> TQAKAKHADVPVNLYRPNAPFIGKVISNEPLVKEGGIGIVQHIKFDLTGGNLKYIEGQSIGIIPPGVDKNGKPEKLRLYSIASTRHGDDVDDKTISLCVRQLEYKHPESGETVYGVCSTYLTHIEPGSEVKITGPVGKEMLLPDDPEANVIMLATGTGIAPMRTYLWRMFKDAERAANPEYQFKGFSWLVFGVPTTPNILYKEELEEIQQKYPDNFRLTYAISREQKNPQGGRMYIQDRVAEHADELWQLIKNQKT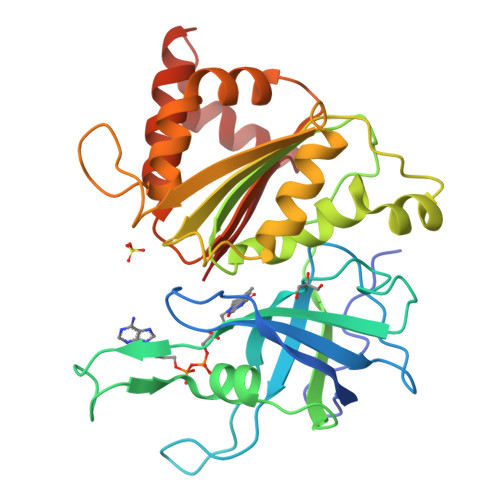HTYICGLRGMEEGIDAALSAAAAKEGVTWSDYQKDLKKAGRWHVETF>LEEKKVCQGTSNKLTQLGTFEDHFLSLQRMFNNCEVVL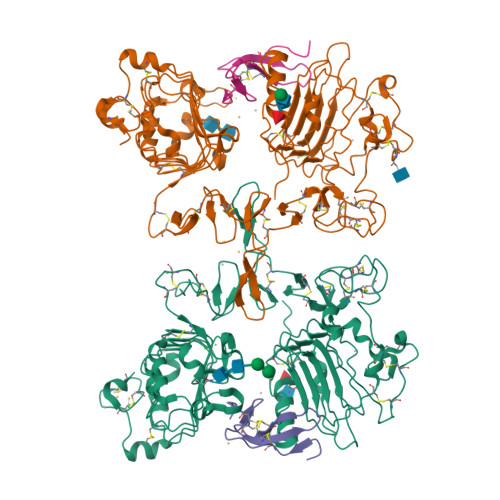GNLEITYVQRNYDLSFLKTIQEVAGYVLIALNTVERIPLENLQIIRGNMYYENSYALAVLSNYDANKTGLKELPMRNLQEILHGAVRFSNNPALCNVESIQWRDIVSSDFLSNMSMDFQNHLGSCQKCDPSCPNGSCWGAGEENCQKLTKIICAQQCSGRCRGKSPSDCCHNQCAAGCTGPRESDCLVCRKFRDEATCKDTCPPLMLYNPTTYQMDVNPEGKYSFGATCVKKCPRNYVVTDHGSCVRACGADSYEMEEDGVRKCKKCEGPCRKVCNGIGIGEFKDSLSINATNIKHFKNCTSISGDLHILPVAFRGDSFTHTPPLDPQELDILKTVKEITGFLLIQAWPENRTDLHAFENLEIIRGRTKQHGQFSLAVVSLNITSLGLRSLKEISDGDVIISGNKNLCYANTINWKKLFGTSGQKTKIISNRGENSCKATGQVCHALCSPEGCWGPEPRDCVS[2x];>VVSHFNDCPDSHTQFCFHGTCRFLVQEDKPACVCHSGYVGARCEHADLLA[2x]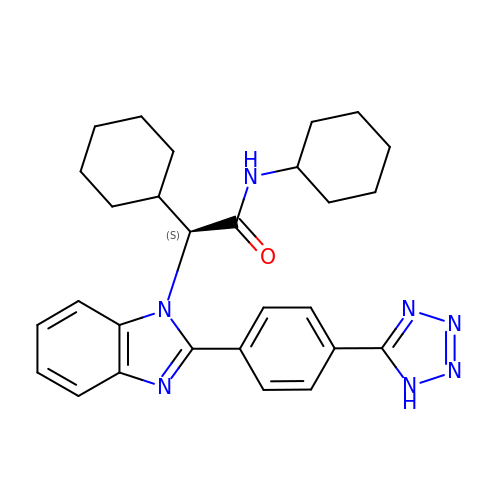(2S)-N,2-dicyclohexyl-2-{2-[4-(1H-tetrazol-5-yl)phenyl]-1H-benzimidazol-1-yl}acetamide | C28 H33 N7 O | WMTZCRYRUZAGRY-VWLOTQADSA-N> AKVGPSKGRGPLLAKFAPVGFKKGFGAIGLGRHTKKGFFIINT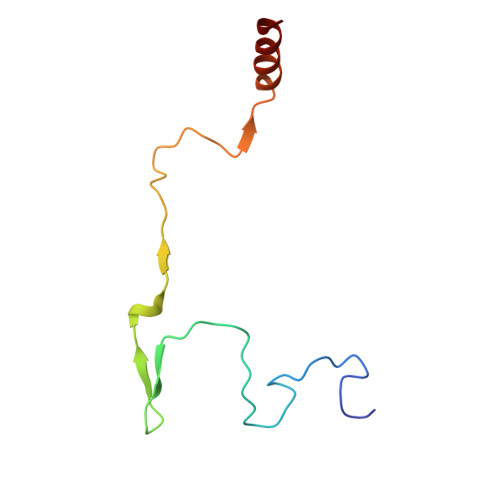MLVPMFKVPDLSNCKLKCYVAPDTYRIVQQSFNKRE>[2x]LLGDFFRKSKEKIGKEFKRIVQRIKDFLRNLVPRTES

Human cathelicidin comprises the cathelin precursor domain and LL-37 as C-terminal extension. LL-37 is activated through proteolytic cleavage as a mature peptide43 comprising 37 amino acids including two N-terminal leucines and a net positive charge of + 6. AMPs in mammals form part of the innate immune response. Their activity includes functions in microbial killing, inflammation, angiogenesis and wound healing.

In our new crystallization attempts of LL-37 in 1% DPC crystals were formed in the presence of 70% MPD. Two antiparallel monomers in the asymmetric unit are crystallographically related to a second dimer, together building a narrow tetrameric 4 nm long channel structure (termed LL-37DPC-4). Notably, this channel does not follow an exact twofold symmetry along the crystallographic channel axis. Disordered residues are observed at both termini resulting in an ordered channel core structure only comprising residues Phe6 to Asn30. Although narrow, the channel shows a continuous and charged inner cavity between the terminal pores with a constriction at the centre. Due to this asymmetric arrangement three different peptide interfaces (IF1, IF2 and IF3) are formed, two of which (IF1) are identical dimer interfaces stabilized by the hydrophobic residues Ile13, Phe17, Ile20, Ile24, Phe27 and Leu31 (interface area 445 Å2—see Fig. 1A). IF1 is further stabilized by two salt bridges involving residues Glu16 and Arg23. The IF2 is stabilized by four hydrophilic residue pairs Lys15/Asn30 and Arg19/Asp26 (contact area 344 Å2). In analogy to IF2 also the smallest interface IF3 is formed by four salt bridges including residues Glu16/Arg23 and Arg19/Asp26 (contact area 339 Å2). In the interior of the channel-like structure a chloride ion is trapped by two Arg23 residues from adjacent monomers and further coordinated by two water molecules.> MSKLVLTGERHYTRNDDIRQSILALGEPGTFMTQDVNIIQTQIEQRLPWIKQVSVRKQWPDELKIHLVEYVPIARWNDQHMVDAEGNTFSVPPERTSKQVLPMLYGPEGSANEVLQGYREMGQMLAKDRFTLKEAAMTARRSWQLTLNNDIKLNLGRGDTMKRLARFVELYPVLQQQAQTDGKRISYVDLRYDSGAAVGWAPLPPEESTQQQNQAQ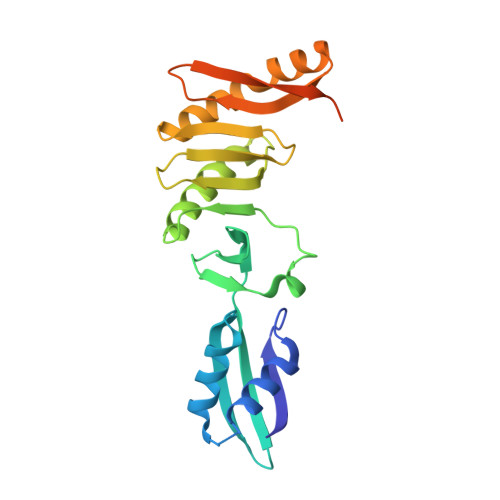AEQQGSHHHHHH>MKNRECCKCYNPCEKICVNYSTTDVAFERPNPCKPTPCKPTPIPCDPCHNTKDNLTGDIVIIGAGAAGSLLAHYLARFSNMKIILLEAGHSHFNDPVVTDPMGFFGKYNPPNENISMSQNPSYSWQGAQEPNTGAYGNRPIIAHGMGFGGSTMINRLNLVVGGRTVFDNDWPVGWKYDDVKNYFRRVLVDINPVRDNTKASITSVALDALRIIAEQQIASGEPVDFLLNKATGNVPNVEKTTPDAVPLNLNDYEGVNSVVAFSSFYMGVNQLSDGNYIRKYAGNTYLNRNYVDENGRGIGKFSGLRVVSDAVVDRIIFKGNRAVGVNYIDREGIMHYVKVNKEVVVTSGAFYTPTILQRSGIGDFTYLSSIGVKNLVYNNPLVGTGLKNHYSPVTITRVHGEPSEVSRFLSNMAANPTNMGFKGLAELGFHRLDPNKPANANTVTYRKYQLMMTAGVGIPAEQQYLSGLSPSSNNLFTLIADDIRFAPEGYIKIGTPNIPRDVPKIFFNTFVTYTPTSAPADQQWPIAQKTLAPLISALLGYDIIYQTLISMNQTARDSGFQVSLEMVYPLNDLIYKLHNGLATYGANWWHYFVPTLVGDDTPAGREFADTLSKLSYYPRVGAHLDSHQGCSCSIGRTVDSNLKVIGTQNVRVADLSAAAFP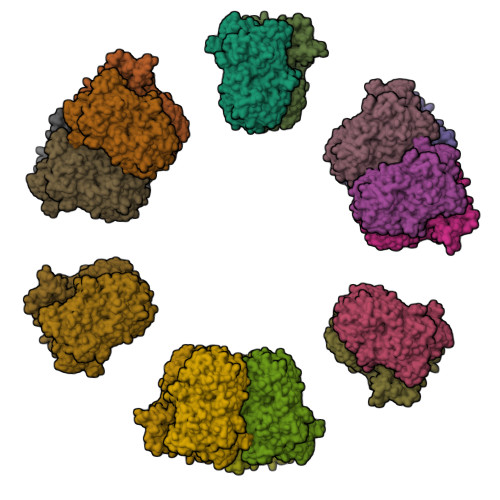PGGNTWATASMIGARAVDLILGFPYLRDLPVNDVPILNVN[2x]> MVHFHPFGGVNFYEMDWSLKGDLWAHDPVIAKEGSRWY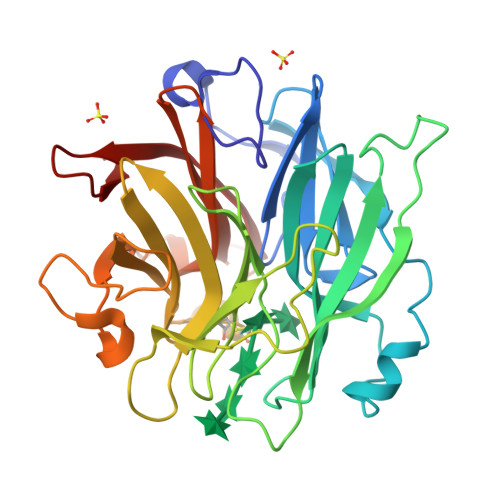VFHTGSGIQIKTSEDGVHWENMGWVFPSLPDWYKQYVPEKDEDHLWAPDICFYNGIYYLYYSVSTFGKNTSVIGLATNQTLDPRDPDYEWKDMGPVIHSTASDNYNAIDPNVVFDQEGQPWLSFGSFWSGIQLIQLDTETMKPAAQAELLTIASRGEEPNAIAAPFIVCRNGYYYLFVSFDFCCRGIESTYKIAVGRSKDITGPYVDKNGVSMMQGGGTILDEGNDRWIGPGHCAVYFSGVSAILVNHAYDALKNGEPTLQIRPLYWDDEGWPYLSV Among the best studied TCSs are the nitrate/nitrite-sensing systems NarX-NarL and NarQ-NarP, responsible for the regulation of anaerobic respiration. NarX phosphorylates NarL in the presence of nitrate and dephosphorylates NarL in its absence; NarQ phosphorylates both NarL and NarP in the presence of nitrate or nitrite and dephosphorylates both proteins in the absence of ligands. Both NarQ and NarX consist of seven domains: a four-helical periplasmic sensor domain, TM bundle, HAMP domain, so-called signaling helix, GAF-like domain, dimerization and histidine phosphotransfer domain, and, finally, catalytic kinase domain. Whereas the sequence identity between NarQ and NarX is ~28%, their ligand binding sites—membrane-proximal parts of the sensor domain’s helices H1 called P boxes—are very well conserved: 14 out of 15 amino acids (residues 42–56 in NarQ) are identical, and the differing ones, Ile45 in NarQ and Lys49 in NarX, are responsible for the differentiation between nitrate and nitrite.

Previous studies of NarX showed that replacing the arginine residue (Arg54, corresponding to Arg50 in NarQ) that coordinates the bound nitrate with lysine or serine resulted in loss of ligand sensitivity and locking of the receptor in the phosphatase state. We obtained the crystals of the R50S mutant of the sensor-TM-HAMP fragment of NarQ using the in meso approach, similarly to our previous work on the wild type protein and its R50K mutant. The crystals diffracted to ~2.0 Å, however the diffraction was anisotropic, and the final dataset was processed to the resolution of 3.3, 2.4, and 2.2 Å along the reciprocal lattice vectors. The crystals belonged to the same space group as the ligand-bound symmetric WT protein, F222. We solved the phase problem using molecular replacement with the structure of the ligand-bound WT sensor-TM-HAMP fragment as a search model. Surprisingly, the backbone of the R50S mutant has the same structure as the ligand-bound WT fragment, despite the Arg→Ser mutation and absence of nitrate in the ligand-binding site. In particular, there is a break in the α-helical structure between TM1 and the helix H1 of the sensor domain, whereas TM2 and the sensor domain helix H4 form a continuous α-helix. A hydrogen bond between Ser50 and Asp133 is observed in the crystal structure of the R50S mutant but not in the MD simulations. MD simulations of the sensor-TM-HAMP fragment of the R50S mutant of NarQ reveal a fast transition to the ligand-free-like conformations, with all of its characteristic features such as diagonal scissoring and formation of a continuous α-helix between H1 and TM1. We conclude that the crystal structure of the R50S is partially artefactual, and the protein is trapped in the ligand-bound-like conformation by crystallization conditions or crystal contacts.

> MIVKRPVSASLARAFFYIVLLSILSTGIALLTLASSLRDAEAINIAGSLSMQSYRLGYDLQSGSPQLNAHRQLFQQALHSPVLTNLNVWYVPEAVKTRYAHLNANWLEMNNRLSKGDLPWYQANINNYVNQIDLFVLALQHYAERKMLLVVAISLAGGIGIFTLVFFTLRRIRHQVVAPLNQLVTASQRIEHGQFDSPPLDTNLPNELGLLAKTFNQMSSELHKLYRSLEHHHHHH> SNAMSNSSMSVVILAAGKGTRMYSDLPKVLHPLAGKPMVQHVIDAAMKLGAQHVHLVYGHGGELLKKTLADPSLNWVLQAEQLGTGHAMQQAAPHFADDEDILMLYGDVPLISVDTLQRLLAAKPEGGIGLLTVKLDNPSGYGRIVRENGDVVGIVEHKDASDAQREINEINTGILVANGRDLKRWLSLLDNNNAQGEFYITDIIALAHADGKKIATVHPTRLSEVEGVNNRLQLSALERVFQTEQAEKLLLAGVMLLDPSRFDLRGELTHGRDITIDTNVIIEGHVILGDRVRIGTGCVLKNCVIGDDSEISPYTVLEDARL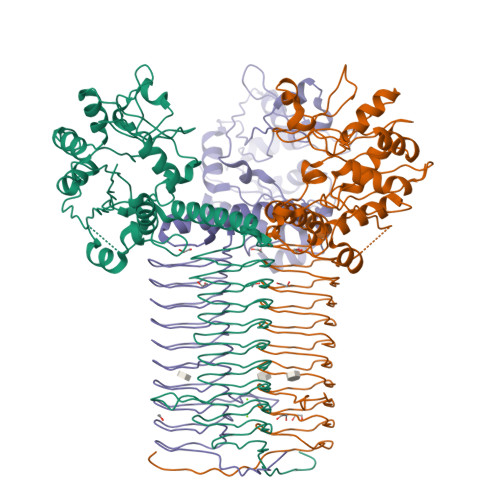DANCTVGPFARLRPGAELAEGAHVGNFVEIKKARLGKGSKAGHLSYLGDAEIGAGVNIGAGTITCNYDGANKFKTIIGDDVFVGSDTQLVAPVTVANGATIGAGTTVTRDVAENELVISRVKQVHIQGWKRPVKKK> MPVDFTGYWKMLVNENFEEYLRALDVN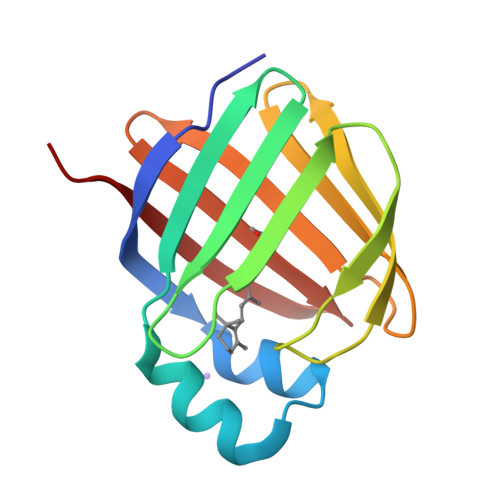VALRKIANLLKPDLEIVQDGDHMIIRTLSTFRNYIMDFQVGKEFEEDLTGIDDRKCMTTVSWDGDKLQCVQKGEKEGRGWTLWIEGDELHLEMRVEGVVCKQVFKKVQ>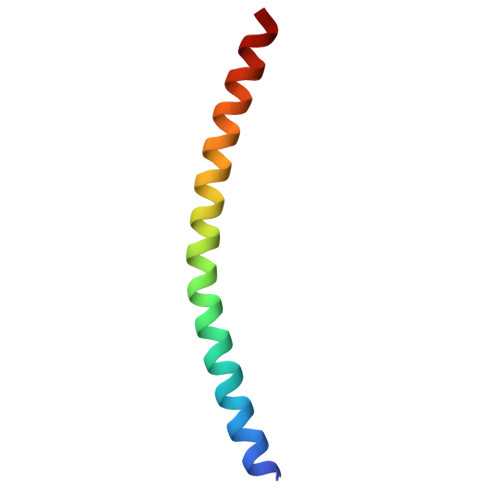 GTYEDLVQAQKEITAHNMQLREQTKQLEHDMAELRDQSQLLLKARCEELK>RLGARPCGLRELEVRV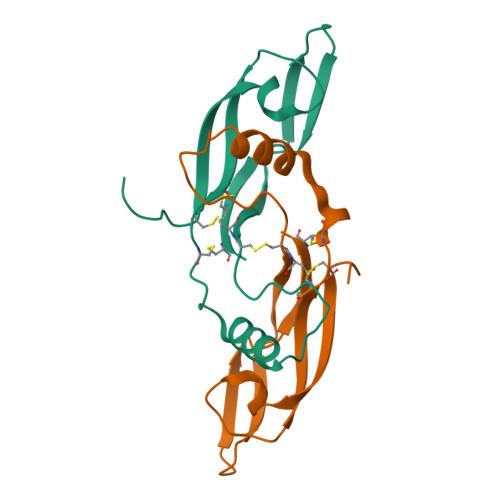SELGLGYASDETVLFRYCAGACEAAARVYDLGLRRLRQRRRLRRERVRAQPCCRPTAYEDEVSFLDAHSRYHTVHELSARECACV[4x]>GAMAQRMVWVDLEMTGLDIEKDQIIEMACLITDSDLNILAEGPNLIIKQPDELLDSMSDWCKEHHGKSGLTKAVKESTITLQQAEYEFLSFVRQQTPPGLCPLAGNSVHEDKKFLDKYMPQFMKHLHYRIIDVSTVKELCRRWYPEEYEFAPKKA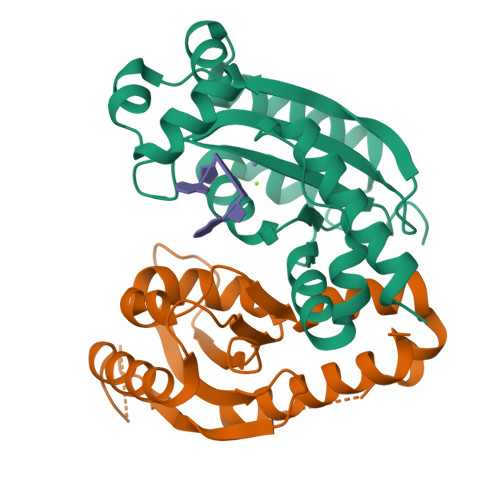ASHRALDAISESIKELQFYRNNIFK[2x]Eukaryotes possess eight highly conserved Lsm (like Sm) proteins that assemble into circular, heteroheptameric complexes, bind RNA, and direct a diverse range of biological processes. Among the many essential functions of Lsm proteins, the cytoplasmic Lsm1–7 complex initiates mRNA decay, while the nuclear Lsm2–8 complex acts as a chaperone for U6 spliceosomal RNA. The Sm family includes the Sm, Lsm (“Like Sm”), and bacterial Hfq proteins. These proteins share a conserved “Sm fold” consisting of an amino-terminal alpha helix followed by five antiparallel beta strands that form small beta barrels that assemble into ring-shaped hexamers or heptamers. Here, we elucidate the molecular basis for Lsm-RNA recognition and present four high-resolution structures of Lsm complexes bound to RNAs.

We crystallized the Lsm2–8 complex bound to UUUUU-3′-OH and UUUUU > p and determined their structures by X-ray diffraction to resolutions of 1.9 and 2.3 Å, respectively. In contrast to the Lsm2–8 complex with unmodified RNA, the structure of the Lsm2–8 ring bound to UUUUU > p reveals that the last nucleotide is highly ordered. The cyclic phosphate causes the RNA chain to make a sharp turn of nearly 180°, which positions the terminal nucleobase to stack over the last histidine at the carboxyl terminus of Lsm8. The terminal uracil base adopts an unusual syn conformation and forms a hydrogen bond to the Lsm3–Asp83 side chain. Lsm3–Arg27 forms a hydrogen bond to a nonbridging oxygen on the terminal cyclic phosphate group and makes a salt bridge with the Lsm8 carboxy-terminal histidine carboxyl group. This binding mechanism is markedly different from that in the S. cerevisiae Lsm2–8 complex with a noncyclic phosphate, where the terminal uridine adopts an anti conformation and lacks direct contacts with the corresponding arginine and aspartate residues (Montemayor et al. 2018). We find that Lsm2–8 binds tightly to an RNA oligonucleotide with a 2′,3′ cyclic phosphate group, and fourfold less tightly to the unmodified RNA with a 3′ hydroxyl (Kd = 26 and 100 nM, respectively). The 2′,3′ cyclic phosphate group bends the RNA chain around and stabilizes an unusual syn conformation of the terminal uracil base. Quantum chemical calculations of 2′,3′ cyclic UMP indicate that the cyclic phosphate stabilizes the syn conformation of uridine to be significantly more favored over the anti conformation. This syn conformation of the terminal uridine facilitates stacking on the Lsm8 carboxy-terminal histidine and allows for a hydrogen bond to Lsm3 Asp83, which could not happen in an anti conformation. The carboxy-terminal histidine residue of Lsm8 that stacks with the terminal syn uracil nucleobase is also strongly conserved in almost all eukaryotes.

>[2x]MLFYSFFKTLIDTEVTVELKNDMSIRGILKSVDQFLNVKLENISVVDASKYPHMAAVKDLFIRGSVVRYVHMSSAYVDTILLADACRRDLANNKRQ;>[2x]GSMESAQAVAEPLDLVRLSLDEIVYVKLRGDRELNGRLHAYDEHLNMVLGDAEEIVTIFDDEETDKDKALKTIRKHYEMLFVRGDSVILIAPPRN;>[2x]MLPLTLLNATQGRPILVELKNGETFNGHLENCDNYMNLTLREVIRTMPDGDKFFRLPECYIRGNNIKYLRIQDEVLSQVAKQQAQQRENRGSRFRGRGQRGRGNYGHTAPNRRGRGRGGHMWSHPQFEK;>[2x]MSMTILPLELIDKCIGSNLWVIMKSEREFAGTLVGFDDYVNIVLKDVTEYDTVTGVTEKHSEMLLNGNGMCMLIPGGKPE;>[2x]GSMDSSPNEFLNKVIGKKVLIRLSSGVDYKGILSCLDGYMNLALERTEEYVNGKKTNVYGDAFIRGNNVLYVSALDD;>[2x]MSSLQKRPGPGNSSQPTERPRKESILDLSRYQDQRIQATFTGGRQITGILKGFDQLMNLVLDDVEEQLRNPEDGKLTGAIRKLGLVVVRGTTLVLIAPMDGSEEIPNPFVQAEHHHHHH;>MSLADFMEQRVQVITNDGRVVLGSLKGFDHTTNLILSDSFERIISMDQDMETIPLGVYLLRGENVAMVGLVNEELDSEIEWTKIRGEAIPDVVH[2x]N~5~-(N-hydroxycarbamimidoyl)-N~5~-methyl-L-ornithine 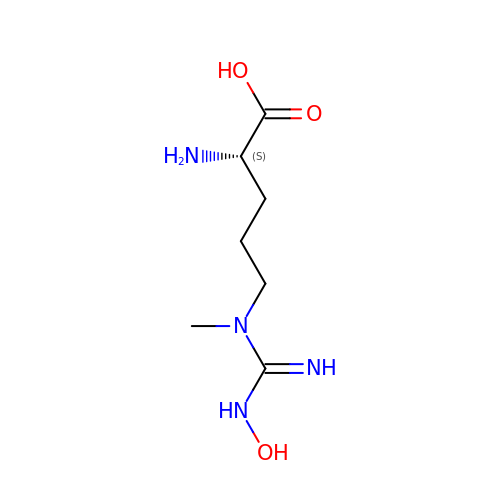| C7 H16 N4 O3 | AUQNEMXAWPGGNP-YFKPBYRVSA-N>SIDVKYIGVKSAYVSYDVQKRTIYLNITNTLNITNNNYYSVEVENITAQVQFSKTVIGKARLNNIT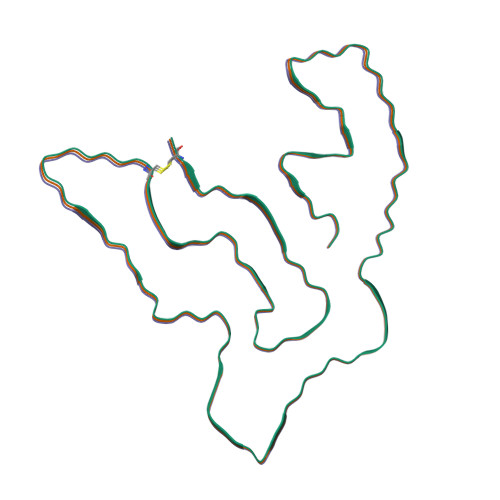IIGPLDMKQIDYTVPTVIAEEMSYMYDFCTLISIKVHNIVLMMQVTVTTTYFGHSEQISQERYQYVDCG[3x]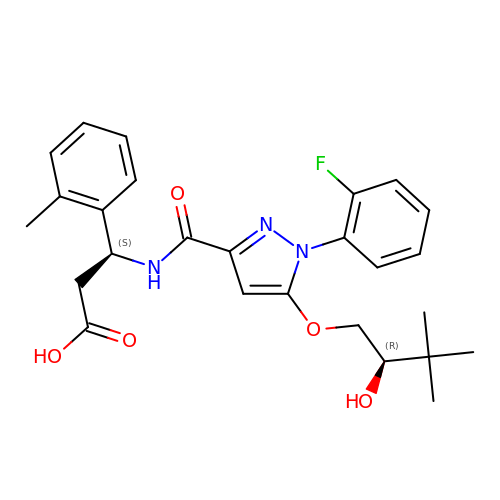(3S)-3-({[1-(2-fluorophenyl)-5-{[(2R)-2-hydroxy-3,3-dimethylbutyl]oxy}-1H-pyrazol-3-yl]carbonyl}amino)-3-(2-methylphenyl)propanoic acid | C26 H30 F N3 O5 | PUJVTKSRQZHCAT-UGKGYDQZSA-N>MTSPSSPPAFRLETSDGGQDGAEVDKAQLGYGAGPPPMESRFQDEDRNFPPQIKVNLNYRKGAGASQPDLNRFDRDRLFNVVARGNPEDLAGLLEYLRRTSKYLTDSEYTEGSTGKTCLMKAVLNLQDGVNACIQPLLEIDRDSGNPQPLVNAQCTDEYYRGHSALHIAIEKRSLQCVKLLVENGANVHAKACGHFFQKNQDTCFYFGELPLSLAACTKQWDVVNYLLENPHQPASLQAQDSLGNTVLHALVMIADDSAENSALVVRMYDGLLQAGARLCPNVQLEGIPNLEGLTPLKLAAKEGKIEIFKHILQREFSAPCQSLSRKFTEWCYGPVRVSLYDLASVDSWEENSVLEIIAFHSRSPHRHRMVVLEPLNKLLQAKWDRLIPRFCFNFLCYLVYMLIFTAVAYHQPALEKQGFPPLKATAGNSMLLLGHILILLGGVYLLLGQLWYFWRRRLFIWISFMDSYSEILFLLQALLTVLSQVLCFLAIEWYLPLLVSSLAMGWTNLLYYTRGFQHTGIYSVMIEKVILRDLLRFLLVYLVFLFGFAVALVSLSREAQNSRTPAGPNATEVGQPGAGQED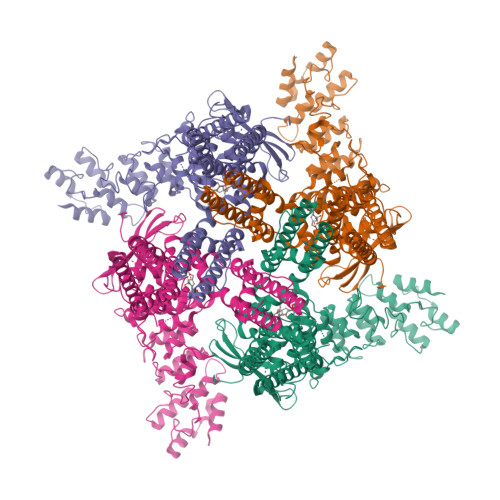EAPPYRSILDASLELFKFTIGMGELAFQEQLRFRGVVLLLLLAYVLLTYVLLLNMLIALMSETVNSVATDSWSIWKLQKAISVLEMENGYWWCRRKKQRAGVMLTVGTRPDGSPDERWCFRVGEMNWATWEQTLPRTLCEEPSGAAAPGVMKNPTPASQRGEDSASEEDHLPLQLLQSRSNLEVLFQGPHHHHHHDYKDDDDK[4x]>[16x]MFGRKKGDVIDAGAELERAEQERIEGEYGASELASERRPHTPGARTLLMVLLCVIAVVLVTLSYKAYKVRGVVEDDDAQPQQVVRQVIPGYTPRPIRPEPENVPEPPQPTTSVPAIQPAPVTQPVRPQPTGPREKTPYELARERMLRSGLTAGSGGGEDLPRPQGGDVPAGGLMGGGGGGGELAEKLQPMRLSGSSAGRLGNRDMLITQGTQLDCVLETRLVTTQPGMTTCHLTRDVYSTSGRVVLLDRGSKVVGFYQGGLRQGQARIFVQWSRIETPSGVVINLDSPGTGPLGEAGLGGWIDRHFWERFGGAIMISLIGDLGDWASRQGSRQGDNSIQFSNTANGVESAAAEALRNSINIPPTLYKNQGERVNILVARDLDFSDVYSLESIPTK;>[16x]MKKLAIVALLASLHAVPALALDVPSSSRYDHRIRYVTYNPADVVQVDTVLGVATHIMLEEGEQYLTHAFGDSEAYAFARKGRHIFIKPQA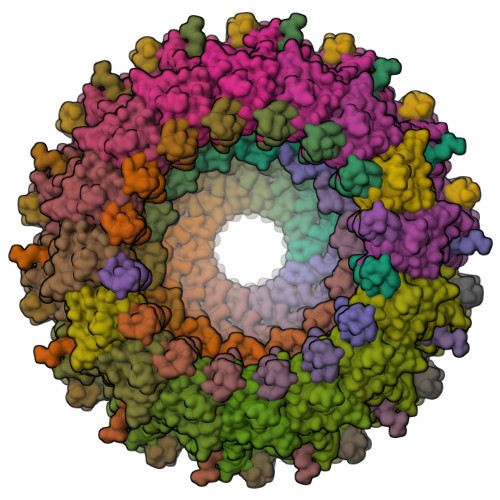ELANTNLIVVTDRRSYKFRLQMRNDRNGAMYELAFRYPDTQARQTREANARAAVEAAFEQRVGAYYNLKYMMSGDKDIAPVNAWDDGRFTYFKFSANADLPSIYFVDAEGNESLVPRTTVGSSNNIIAVHKVNPKWMIRLGNRALAIFNEAYDPNGVPNDTGTASPAVRRVNKGGN;>MKTIIFAILMTGLLSACASAPKPKQPSDFNREPVNKTVPVEIQRGAL[14x]4-[[(4~{S},5~{R})-4,5-bis(4-chlorophenyl)-2-(4-methoxy-2-propan-2-yloxy-phenyl)-4,5-dihydroimidazol-1-yl]carbonyl]-3-methylidene-piperazin-2-one | C31 H30 Cl2 N4 O4 | 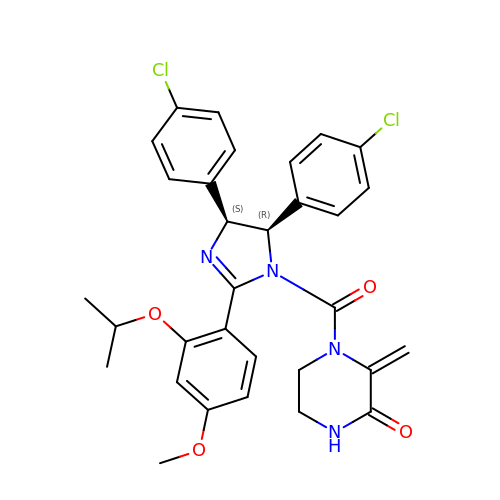JLTUTZCZAIJXTD-WUFINQPMSA-N>[2x]MAKSKAAAAAPALQGDVPGRLAGKIAVVTGAAGNLGGHIVTHYLAEGATVVMTGRTPDRTKAAADALLKSTGADPSRLATVALDGGDIASVRAAIAEVVQKFGRIDILVNNAGSAGPKQPIENLPLSPEELAALQKTGSTDSETVADALRNIFGVAWNVARVAAPHIPEGGSIINVSTIFSRTPYYARAAYVVPKAAMNAWSRELSLELGPKGIRVNLVYPGPIESERIRSVFAAMDAARGDEAGTTATQFFDMMSLERATGGNEKAKTFPTPEDIATTCVFLGSDESAAYNGHDFEVTHGMSVRKEQRSTYLARPTMRSMDGTGLAVLIAAGDDWEEALEIAQVQLACGAQVVLGLPRAADVAIAEKRCKALGLTEGLSIIRFSR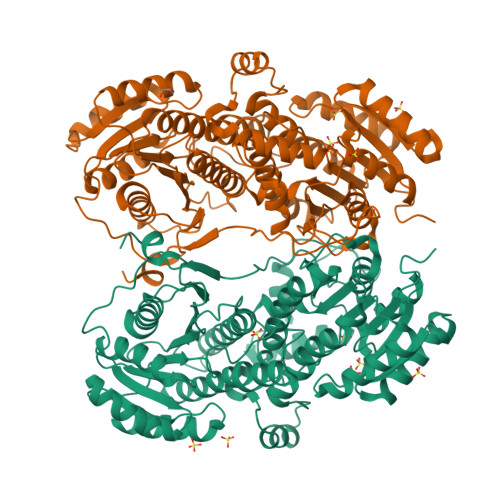KDPAAMEAALEEYTRGGTPISGALFMPALGAGELSGAVTEAEDNAVEALMDAELAGNMALARTMSRYWKRHDNLLQPPRFVFVSHASDGKGDIYGHILRAATEQLIRIWRDESEIDTAHGRRRQAEWGNQIVRFTNTEAENIRFTAGHAARILLKESKLGEITLYVPANIGEATGARKAMPLEHHHHHH BlaR1 and MecR1 are membrane proteins with an N-terminal zinc metalloprotease domain and a C-terminal extracellular β-lactam-binding sensor domain. β-Lactam binding to the extracellular BlaR1 sensor domain regulates BlaI cleavage by the zinc metalloprotease domain in the cytoplasm. BlaR1 forms a domain-swapped dimer, with the zinc metalloprotease active site accessible from the cytoplasm. BlaR1 undergoes spontaneous autocleavage in cis between Ser283 and Phe284 and we describe the catalytic mechanism and specificity underlying the self and BlaI cleavage.

BlaR1 was consistently observed in a dimeric form with two-fold symmetry averaging applied in the overall reconstructions for each sample. More structural heterogeneity was detected in the BlaR1(WT) dataset compared with the uncleavable mutant BlaR1(F284A), suggesting enhanced dynamic motions. In the BlaR1(WT) dataset, the sensor domains were observed to be dynamic and are able to adopt different orientations with respect to each other and the transmembrane domains. A comparison with BlaR1(F284A) shows that the sensor domains are positioned at different distances to the transmembrane domain in order of BlaR1(WT), BlaR1(F284A) and BlaR1(F284A)–ampicillin. Although a range of states exists in all of the samples, the equilibrium is shifted—BlaR1(WT) is dominated by a more extended conformation and the BlaR1(F284A)–ampicillin structure is more compact, with the sensor directly in contact with the outer leaflet of the membrane. In the BlaR1(F284A) mutant structures, the autocleavage loop is intact; however, in the BlaR1(WT) structure, we detected a mixture of uncleaved and cleaved forms, the latter with the central P1′ Phe284 slightly shifted in position. Here, BlaR1(WT) undergoes spontaneous autocleavage, consistent with previous reports. In all of the structures, the protease domain is in an autoinhibited state with the autocleavage loop (both cleaved and uncleaved) occupying the active site, suggesting an equilibrium between active site occupied/autoinhibited and active site accessible states.

>MAKLLIMSIVSFCFIFLLLLFFRYILKRYFNYMLNYKVWYLTLLAGLIPFIPIKFSLFKFNNVNNQAPTVESKSHDLNHNINTTKPIQEFATDIHKFNWDSIDNICTVIWIVLVIILSFKFLKALLYLKYLKKQSLYLNENEKNKIDTILFNHQYKKNIVIRKAETIQSPITFWYGKYIILIPSSYFKSVIDKRLKYIILHEYAHAKNRDTLHLIIFNIFSIIMSYNPLVHIVKRKIIHDNEVEADRFVLNNINKNEFKTYAESIMDSVLNVPFFNKNILSHSFNGKKSLLKRRLINIKEANLKKQSKLILIFICIFTFLLMVIQSQFLMGQSITDYNYKKPLHNDYQILDKSKIFGSNSGSFVMYSMKKDKYYIYNEKESRKRYSPNSTYKIYLAMFGLDRHIINDENSRMSWNHKHYPFDAWNKEQDLNTAMQNSVNWYFERISDQIPKNYTATQLKQLNYGNKNLGSYKSYWMEDSLKISNLEQVIVFKNMMEQNNHFSKKAKNQLSSSLLIKKNEKYELYGKTGTGIVNGKYNNGWFVGYVITNHDKYYFATHLSDGKPSGKNAELISEKILKEMGVLNGQELALVPRGSSAHHHHHH[2x]> TVPDNLKKQLAVSVRNIQWSYGIFWSVSASQPGVLEWGDGYYNGDIKTRKTIQAAEVKIDQLGLERSEQLRELYESLSLAESSASGSSQVTRRASAAALSPEDLTDTEWYYLVCMSFVFNIGEGIPGGALSNGEPIWLCNAETADSK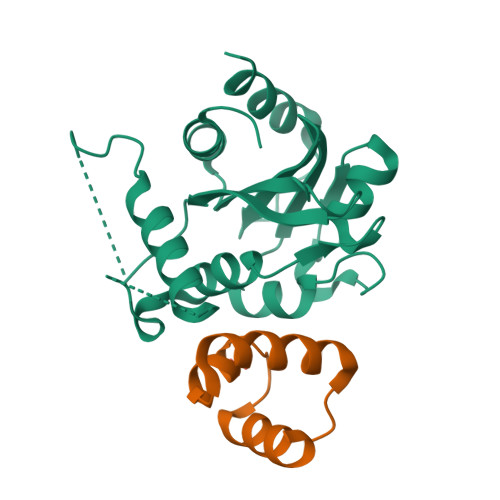VFTRSLLAKSASLQTVVCFPFLGGVLEIGTTEHIKEDMNVIQSVKTLFLEA;> VKMSEEEEDLISRMYKLVGDRWELIAGRIPGRTPEEIERYWLMKHGVVFANRRRDFFRK> MHHHHHHSSGLVPRGSPQYGIAREDVVLNRILGEGFFGEVYEGVYTNHKGEKINVAVKTCKKDC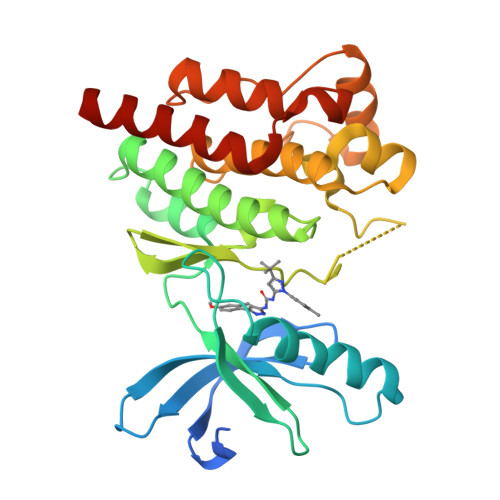TLDNKEKFMSEAVIMKNLDHPHIVKLIGIIEEEPTWIIMELYPYGELGHYLERNKNSLKVLTLVLYSLQICKAMAYLESINCVHRDIAVRNILVASPECVKLGDFGLSRYIEDEDYYKASVTRLPIKWMSPESINFRRFTTASDVWMFAVCMWEILSFGKQPFFWLENKDVIGVLEKGDRLPKPDLCPPVLYTLMTRCWDYDPSDRPRFTELVCSLSDVYQMEKDIAME> MSKIVAVVVLAAFCVAMLV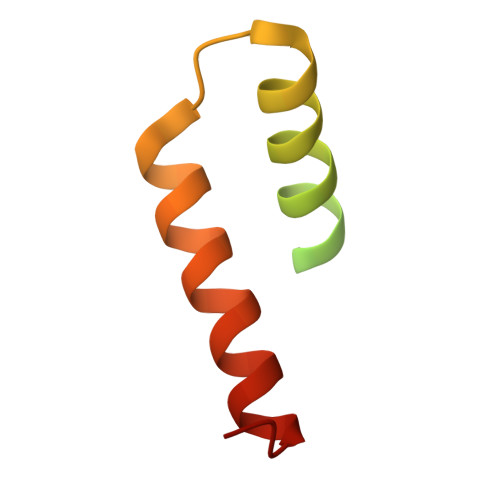SDVSAKTSISVKGESNVDVVSQINSLVSSIVSGANVSAVLLAQTLVNILQILIDANVFA> MDIGIDSDPQKTNAVPRPKLVVGLVVDQMRWDYLYRYYSKYGEGGFKRMLNTGYSLNNVHIDYVPTVTAIGHTSIFTGSVPSIHGIAGNDWYDKELGKSVYCTSDETVQPVGTTSNSVGQHSPRNLWSTTVTDQLGLATNFTSKVVGVSLKDRASILPAGHNPTGAFWFDDTTGKFITSTYYTKELPKWVNDFNNKNVPAQLVANGWNTLLPINQYTESSEDNVEWEGLLGSKKTPTFPYTDLAKDYEAKKGLIRTTPFGNTLTLQMADAAIDGNQMGVDDITDFLTVNLASTDY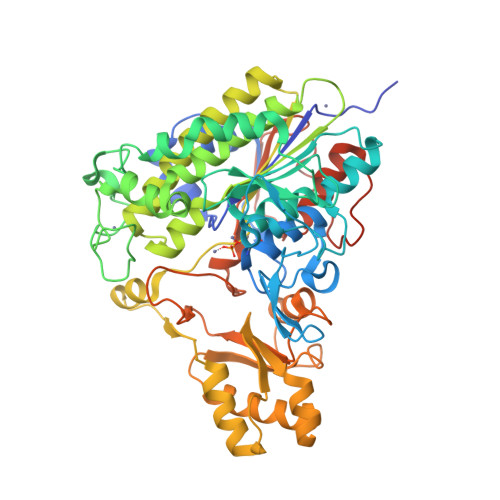VGHNFGPNSIEVEDTYLRLDRDLADFFNNLDKKVGKGNYLVFLSADHGAAHSVGFMQAHKMPTGFFVEDMKKEMNAKLKQKFGADNIIAAAMNYQVYFDRKVLADSKLELDDVRDYVMTELKKEPSVLYVLSTDEIWESSIPEPIKSRVINGYNWKRSGDIQIISKDGYLSAYSKKGTTHSVWNSYDSHIPLLFMGWGIKQGESNQPYHMTDIAPTVSSLLKIQFPSGAVGKPITEVIGRIEGRSAWSHPQFEK>AEEELPPRKVCIVGA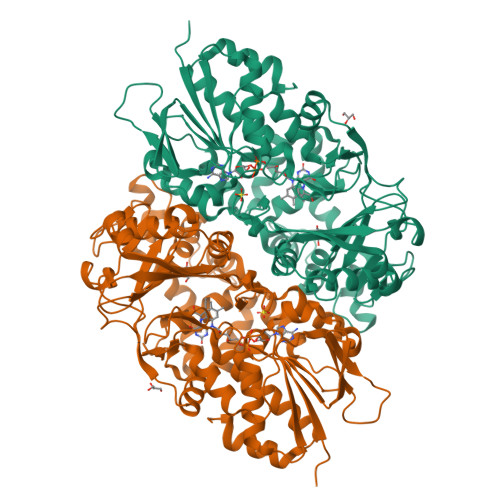GVSGLYIAMILDDLKIPNLTYDIFESSSRTGGRLYTHHFTDAKHDYYDIGAMRYPDIPSMKRTFNLFKRTGMPLIKYYLDGENTPQLYNNHFFAKGVVDPYMVSVANGGTVPDDVVDSVGEKLQQAFGYYKEKLAEDFDKGFDELMLVDDMTTREYLKRGGPKGEAPKYDFFAIQWMETQNTGTNLFDQAFSESVIASFDFDNPTKPEWYCIEGGTSLLVDAMKETLVHKVQNNKRVEAISIDLDAPDDGNMSVKIGGKDYSGYSTVFNTTALGCLDRMDLRGLNLHPTQADAIRCLHYANSTKVALKFSYPWWIKDCGITCGGAASTDLPLRTCVYPSYNLGDTGEAVLLASYTWSQDATRIGSLVKDAPPQPPKEDELVELILQNLARLHAEHMTYEKIKEAYTGVYHAYCWANDPNVGGAFALFGPGQFSNLYPYLMRPAAGGKFHIVGEASSVHHAWIIGSLESAYTAVYQFLYKYKMWDYLRLLLERWQYGLQELETGKHGTAHLQFILGSLPKEYQVKI[2x]>[2x]MSDPSAKPLQEHILIILDDAGRREVLLTETFYTIGRSPRADIRIKSQFVSRIHAVLVRKSSDDVQAAYRIIDGDEDGQSSVNGLMINGKKVQEHIIQTGDEIVMGPQVSVRYEY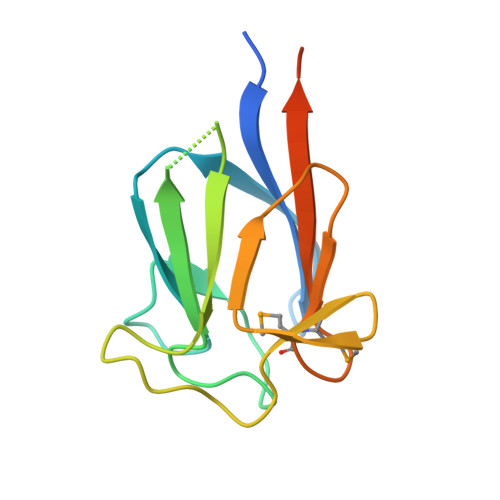RRRDQFGTMLEHHHHHH>[10x]GWGQPHGGGWGQGGGTHSQWNKPSKPKTNMKHMAGAAAAGAVVGGLGGYVLGSAMSRPIIHF

Prion protein (PrP) aggregation and formation of PrP amyloid (APrP) are central events in the pathogenesis of prion diseases. The c.593t > c mutation in the prion protein gene (PRNP) results in a phenylalanine to serine amino acid substitution at PrP residue 198 (F198S) and causes the most severe amyloidosis among GSS variants. Using cryogenic electron microscopy (cryo-EM), we determined for the first time the structures of filaments of human APrP, isolated post-mortem from the brain of two symptomatic PRNP F198S mutation carriers. The protomers in the cross-β spines consist of 62 amino acids and span from glycine 80 to phenylalanine 141, adopting a previously unseen spiral fold with a thicker outer layer and a thinner inner layer.

We report that in GSS (F198S) APrP filaments are composed of dimeric, trimeric and tetrameric left-handed protofilaments with their protomers sharing a common protein fold. Each protomer comprises nine short β-strands, with the β1 and β8 strands, as well as the β4 and β9 strands, forming a steric zipper. APrP deposits in GSS (F198S) are composed of N- and C-terminally truncated fragments of PrP, formed through proteolytic cleavage of the precursor protein. It has been previously shown that the fragments vary in lengths and span approximately from residues G58 to E152. The sequence of the APrP forming peptides does not include the F198S mutation, glycans or the glycosylphosphatidylinositol (GPI)-anchor.4-[(5-methyl[1,2,4]triazolo[1,5-a]pyrimidin-7-yl)amino]phenol 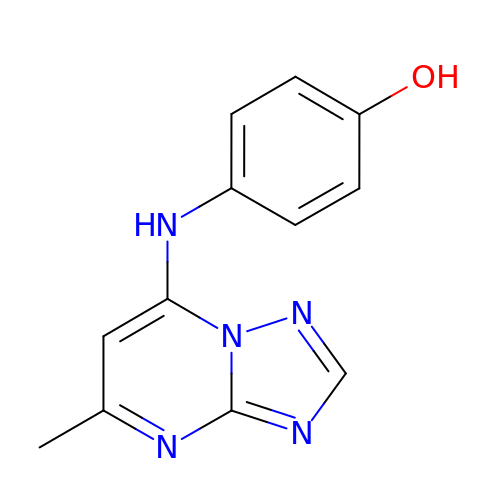| C12 H11 N5 O | QHEXWJVMHICYCY-UHFFFAOYSA-N Prototypical phytochromes can exist in two photochemical states with differential cellular signaling activity, called red light-absorbing (Pr) and far-red light-absorbing (Pfr) state. Light is detected by a bilin chromophore, which is covalently linked to the photosensory core of the protein, comprising of PAS (Per/Arndt/Sim), GAF (cGMP phosphodiesterase/adenyl cyclase/FhlA) and PHY (phytochrome-specific) domains. Important for the signaling is a stretch of amino acids in the PHY domain, called the PHY-tongue, which changes from a β-sheet in Pr into an α-helix in Pfr state (Essen et al., 2008; Yang et al., 2008; Takala et al., 2014; Sanchez et al., 2019) The chromophore connects to the PHY-tongue via a strictly conserved aspartatic acid, which is expected to play a crucial role in signal transduction. To address this gap of knowledge, we recorded time-resolved serial femtosecond X-ray crystallographic (SFX) data of the PAS-GAF domains of the phytochrome from Deinococcus radiodurans (DrBphPCBD) at 1 ps and 10 ps after femtosecond optical excitation.

Two propionate side chains additionally anchor the chromophore non-covalently to the protein. The pyrrole water is ubiquitously found in phytochrome structures. The strictly conserved Asp207 is a key residue for signal transduction because it connects the chromophore to the PHY-tongue in Pr and Pfr. The A-ring is covalently attached to the protein backbone in phytochromes, which renders complete isomerization impossible, but is sufficiently flexible to accommodate the proposed changes.

>MASMTGGQQMGRGSMSRDPLPFFPPLYLGGPEITTENCEREPIHIPGSIQPHGALLTADGHSGEVLQMSLNAATFLGQEPTVLRGQTLAALLPEQWPALQAALPPGCPDALQYRATLDWPAAGHLSLTVHRVGELLILEFEPTEAWDSTGPHALRNAMFALESAPNLRALAEVATQTVRELTGFDRVMLYKFAPDATGEVIAEARREGLHAFLGHRFPASDIPAQARALYTRHLLRLTADTRAAAVPLDPVLNPQTNAPTPLGGAVLRATSPMHMQYLRNMGVGSSLSVSVVVGGQLWGLIACHHQTPYVLPPDLRTTLEYLGRLLSLQVQVKEALEHHHHHH[2x]> GSSMANNALQTIINARLPGEEGLWQIHLQDGKISAIDAQSGVMPITENSLDAEQGLVIPPFVEPHIHLDTTQTAGQPNWNQSGTLFEGIERWAERKALLTHDDVKQRAWQTLKWQIANGIQHVRTHVDVSDATLTALKAMLEVKQEVAPWIDLQIVAFPQEGILSYPNGEALLEEALR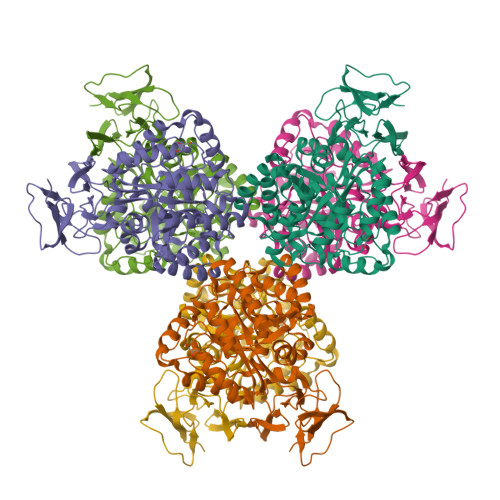LGADVVGAIPHFEFTREYGVESLHKTFALAQKYDRLIDVHCDEIDDEQSRFVETVAALAHHEGMGARVTASHTTAMHSYNGAYTSRLFRLLKMSGINFVANPLVNIHLQGRFDTYPKRRGITRVKEMLESGINVCFGHDGVFDPWYPLGTANMLQVLHMGLHVCQLMGYGQINDGLNLITHHSARTLNLQDYGIAAGNSANLIILPAENGFDALRRQVPVRYSVRGGKVIASTQPAQTTVYLEQPEAIDYKR>MAKLRVGIVFGGKSAEHEVSLQSAKNIVDAIDKTRFDVVLLGIDKAGQWHVNDAENYLQNADDPAHIALRPSAISLA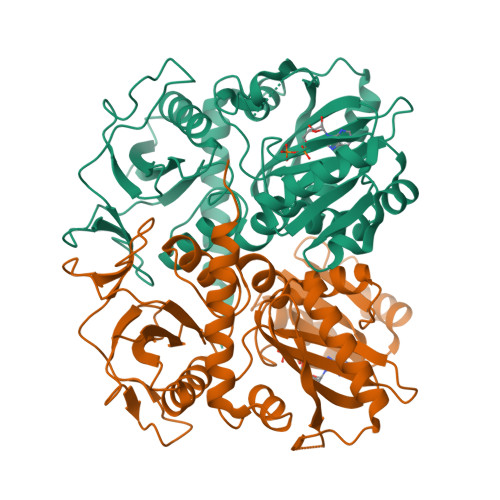QVPGKHQHQLINAQNGQPLPTVDVIFPIVHGTLGEDGSLQGMLRVANLPFVGSDVLSSAACMDKDVAKRLLRDAGLNIAPFITLTRTNRHAFSFAEVESRLGLPLFVKPANQGSSVGVSKVANEAQYQQAVALAFEFDHKVVVEQGIKGREIECAVLGNDNPQASTCGEIVLNSEFYAYDTKYIDDNGAQVVVPAQIPSEVNDKIRAIAIQAYQTLGCAGMARVDVFLTADNEVVINEINTLPGFTNISMYPKLWQASGLGYTDLISRLIELALERHTANNALKTTM[4x]> SNALHLEPLHFLQCHSRNNSPKDLETQLWACAFEPAREEGHSGATSQTVATCGGEAVCVIDCQTGLVLHKYKVPGEEFFSVAWTALTVATQAGHKKRWNMLAAAGLRG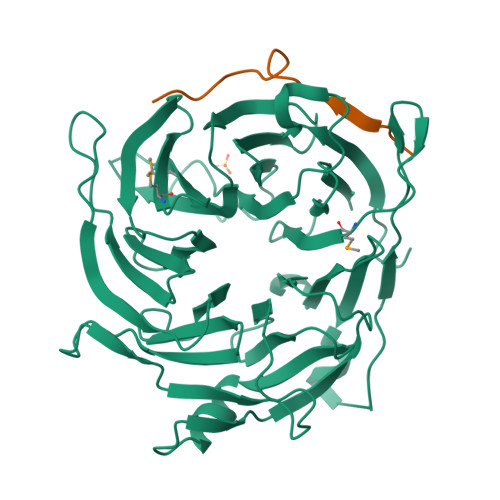MVRLLHVRAGFCCSVIRAHKKAIATLCFSPTHETHLFTASYDKRIILWDIGVPNHDYKFQASQLLTLNCSSVPLRLCPVATCPDSFLLAGCEGGCGCWDVRLDQPQKQRVCEVNFVFSGDSEVSGQRVDGLAFVNEDVVASKGSGQGTIYLWSWSQTWASRGSQSVLPVVILAQLQWSPTSLAYFSLSTCPDKNLVLCGDEEGSVWIYDVEHLLKQPPPLETTLQPPTQILKWPQPVALGQPVTKTMVNTVVANAAFTYLTALTDSNIVSIWRRC;> SNAMSTLRLKEAKVPSVQFVGDDDVLSHILDREGGTKLKKEKVQLLVNPQKVIKKAECELEKSDLEVLEDQNYVEVLGRNIQESLGNGSAVDGRNKVYSFQHR>GKLYLNHSAKQHTSASDHLLTEISVNHGEHKQVTLPDGTVVHLNAGTVMRYPTEFTSDIRLVEMEGEAFFNVMRDEGKPFIVRTRQADVKVLGGSFNVKAYQEDELMAVSVRTGKVEVDMPESVMRLLPNEQIIVNNTNGEILKKNEDAQKVTAW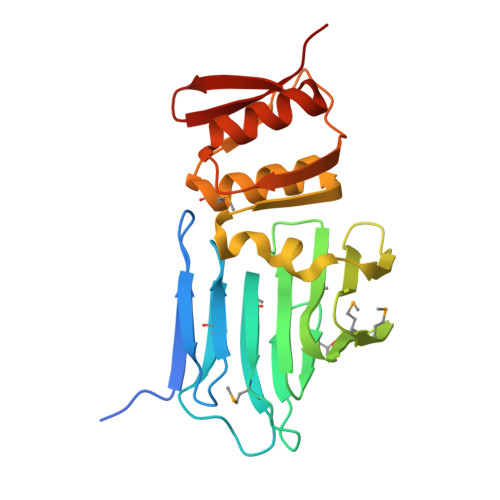LQGGLYFNRTPISSVIHDLERMYNQEIVLDPNVVFDDYIYGEHDNKSLEAVLNAIQYSTGIRYRKEESRIVLYKTSH[2x]Gene transfer agents (GTAs) are DNA-containing phage-like particles produced by some species of bacteria and archaea. The genes encoding proteins that form Rhodobacter capsulatus GTA particles (RcGTA) are derived from phage DNA, which has been integrated into the bacterial genome. Here, we use cryo-electron microscopy (cryo-EM) to determine the structures of RcGTA before and after DNA ejection, and to visualize the interactions of RcGTA with R. capsulatus cells. Particles of RcGTA have heads with a diameter of 38-nm and 49-nm long tails.

The dodecamer of the adaptor proteins provides the binding site for a hexamer of stopper proteins, resulting in a symmetry mismatch between the two complexes. Adaptor loops from two neighboring adaptor proteins differ in their conformations and interact with one subunit of stopper protein. The first adaptor loop is oriented parallel to the tail axis and fits into a cleft within β-sheets of a stopper protein, whereas the adaptor loop of the second subunit is wedged between two stopper proteins. A hexamer of RcGTA stopper proteins (Rcc01689, g7) binds to the adaptor complex. Each 112-residue-long stopper protein interacts with adaptor loops from two neighboring adaptor proteins. At the distal interface, the long and insertion loops and C-terminus of the stopper protein bind to a terminator protein. However, the long loop of the RcGTA stopper protein interacts with the tail terminator protein and does not block the central tail channel. Furthermore, the end of the DNA packaged in the native RcGTA particle extends through the channel formed by the hexamer of stopper proteins and continues into the disc of tail terminator proteins. A hexamer of tail terminator proteins (Rcc01690, g8) binds to the distal interface of the stopper proteins. Unlike other tail proteins of RcGTA, the tail terminator protein contains α-helices 1 and 2 in its N-terminus. α-helix 1 binds to the insertion loop of the stopper protein and α-helix 2 interacts with α-helix 3 from the same tail terminator protein.

>MGLNFFRKAAPEVRTEPVAERKASVTGRIVAMASGAGRPVWGPRDTVSLMRTGFAGNPVGFRSVKLIAEATAAVPLICQDAERRYEIHPVLDLLRRPNAGQGRAELFEALIGQILLSGNGYLEAVCPEPGVPRELHVLRSDRMAVVPGADGWPVGYDYTVGGRKHRFDMTGHPDPICHIKSFHPTDDHYGLSPMQAAAVALDVHNAASAWSKALLDNAARPSGAIIYKGADGQGVLAPEQYERLIFEMETHHQGARNAGRPMLLEGGLDWKPMGFSPSDMEFHETKAAAAREIALAFGVPPMLIGIPGDATYANYAEANRAFYRLTVLPLLTRVSAALAWWLSGYLGAQIELKPDLDQVPALAVERDQLWARIGAAGFLSNSEKRVLLGLPPTAEG[2x];>MMLNEVTAVPGTALPVAEFRDHLRLGTGFADLGAEDAALLSYLRAAIAAIEGRTAKALISRGFRLALTAWRWGDMQTLPIAPVATVTALRLVDAAGVETPVAAGWRLVPDMARPRIEALGAMLPMIPTGGRVEIDFTAGFGASWSALPVDLAQAVFLLAAQYYELRHDGAAEGGAMPFGVMALIERWRTVRVLGGRP[2x];> MSRPRLNRLLVLEEAVRVADGAGGHRLDWQAKGEVWAEVTAGSGSERAGEFVTLASVPFTIVVRAAPVGAARRPRPEQRFREGARIFRILAVAERDREGHYLSCFAREEVVA;> MSYAVAGALQAAVYQQLRADAVLAALVGTAVYDAVPPGPLAGTYVSLGPEDVADASDKTGAGAVHDFVISVITDAAGFATAKAAAAAVSDALVGADLVLSRGRLVGLWFLRAKARRVEKADMRRIDLVFRARVEG;> MAAQNGKDLLIKLDLTGSGQFETIAGLRATRISFNAETVDVTSLESQGGWRELLGGAGVRSASISGAGVFKDADTDERARQIFFDGEVPEFQVIIPDFGIVQGPFMITSIDYAGSHNGEASYELAMASAGALSFTAI Ricin consists of a toxic subunit, known as the A chain (RTA), and a subunit that binds galactose and N-acetylgalactosamine, known as the B chain (RTB)3. RTA has a molecular mass of 30 kDa and exhibits RNA N-glycosidase activity, which inactivates ribosomes by removing the A4324 in the sarcin-ricin loop of 28 S rRNA4. Eukaryotic ribosomal P stalk proteins have been proven to be essential for RTA binding and rRNA depurination. A distinctive feature of P stalk proteins is that they contain a highly conserved set of 11 residues (SDDDMGFGLFD) at the C-terminal tail of P2 that recruits elongation factors and interacts with several RIPs, such as trichosanthin and Shiga toxin 11415.

To promote a more efficient interaction between RTA and the synthetic C10-P2 peptide, we constructed a chimeric protein in which C10-P2 was fused to the C-terminus of RTA using four consecutive Gly-Ser (GS) repeats as a linker. Finally, we determined the structure of the RTA-C10-P2 fusion protein at a resolution of 1.5 Å. For the C10-P2 peptide, only 6 residues (GFGLFD) could be fitted to the observed electron density; these residues corresponded to Gly110-Asp115 of the human P2 protein. The 4 N-terminal residues (DDDM) were disordered and did not seem to contribute to RTA binding. As shown in Fig. 2 (A,B), the C-terminus of C10-P2 is coiled into a short helix that binds in a pocket formed by α6, α7, α8, β7 and β8 of RTA. The root mean square deviation (RMSD) of the overall main chain of the RTA moiety in RTA-C10-P2 and wild-type RTA is 0.290 Å for 222 comparable Cα atoms, indicating that the binding of C10-P2 does not substantially affect the structure of RTA. The Gly110 and Gly112 residues of P2 accommodate the required backbone dihedral angles to facilitate the insertion of Phe111, Leu113 and Phe114 into a hydrophobic pocket formed by the Tyr183, Arg235, Phe240 and Ile251 residues of RTA. The main-chain carbonyl of Phe114 in P2 forms a hydrogen bond with the main-chain amide of Arg235 in RTA, and the side-chain atom OD1 of Asp115 in P2 forms another hydrogen bond with the side-chain atom NE of Arg235 in RTA. When these 16 residues form a β-strand, the length of this strand is predicted to be 56 Å, which is much longer than 29 Å. Based on the above considerations, we believe that the linker may adopt a flexible conformation of sufficient length and thus does not disturb the interaction between the P2 peptide and RTA.

> MGHHHHHHIFPKQYPIINFTTAGATVQSYTNFIRAVRGRLTTGADVRHEIPVLPNRVGLPINQRFILVELSNHAELSVTLALDVTNAYVVGYRAGNSAYFFHPDNQEDAEAITHLFTDVQNRYTFAFGGNYDRLEQLAGNLRENIELGNGPLEEAISALYYYSTGGTQLPTLARSFIICIQMISEAARFQYIEGEMRTRIRYNRRSAPDPSVITLENSWGRLSTAIQESNQGAFASPIQLQRRNGSKFSVYDVSILIPIIALMVYRCAPPPSSQF;> DDDMGFGLFD> MSGEKGYWFELPVPALLPLPNGYAIISEFGEHYPRKQAGNDWFVVDPASVSLPLRVRTRRRGDRMVLKGTGGTKKLKEIFIEAKIPRMERDRWPIVEDADGRILWVPGLKKSAFEAQNRGQARYILLQYQAMN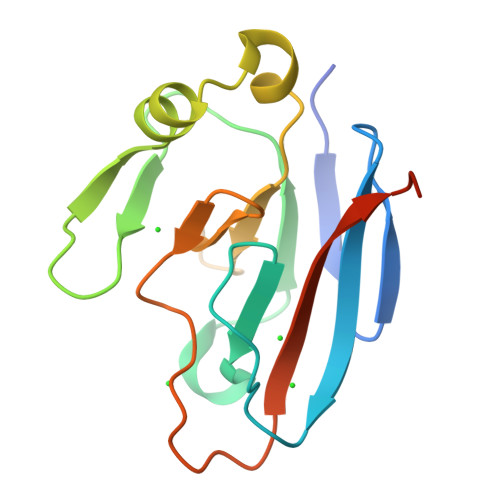SLEHHHHHH>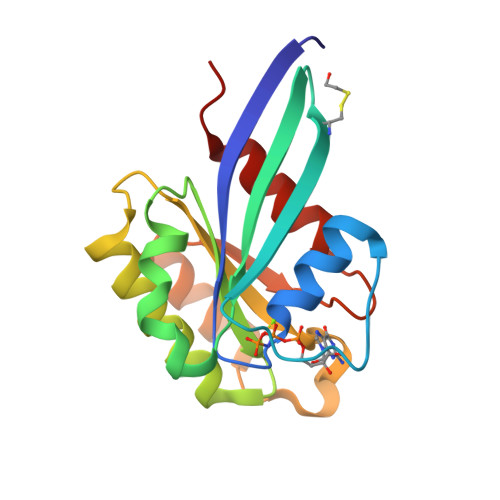 GNKICQFKLVLLGESKVGKSSLVLRFVKGQFHEFQESTIGAAFLTQTVCLDDTTVKFEIWDTAGQERYHSLAPMYYRGAQAAIVVYDITNEESFARAKNWVKELQRQASPNIVIALSGNKADLANKRAVDFQEAQSYADDNSLLFMETSAKTSMNVNEIFMAIAKKLPKN> MHYELSAAARAAFLSKYRDFPHYMENRNFTPPKDGGMWLRFNYIEGDTLYLSIDRKCKSYIAIVQIGVVFPPGSGVDEARLKAKEIAD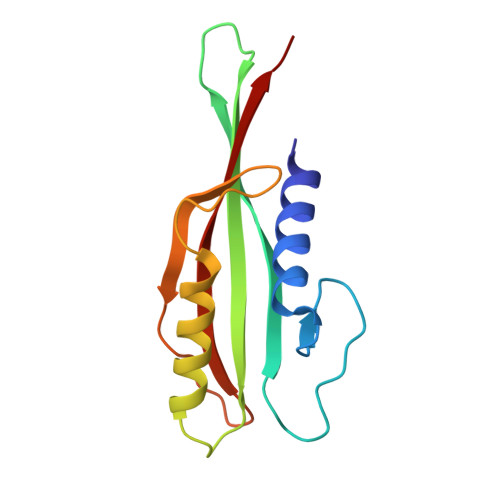FFKDGKMLNVGYIFEGAIVHQIVKHESGWMIPVRFTVRVDTKET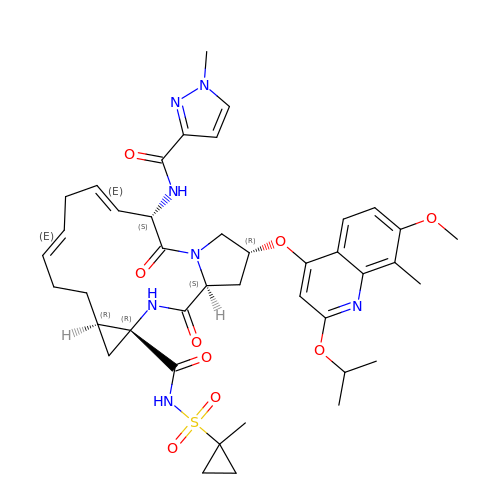(2R,6S,7E,10E,13aR,14aR,16aS)-2-{[7-methoxy-8-methyl-2-(propan-2-yloxy)quinolin-4-yl]oxy}-N-[(1-methylcyclopropyl)sulfonyl]-6-{[(1-methyl-1H-pyrazol-3-yl)carbonyl]amino}-5,16-dioxo-1,2,3,6,9,12,13,13a,14,15,16,16a-dodecahydrocyclopropa[e]pyrrolo[1,2-a][1,4]diazacyclopentadecine-14a(5H)-carboxamide | C41 H51 N7 O9 S | ZHIQOLBHZJFLCW-QVARATBXSA-N(2~{S},3~{S},4~{R},5~{R})-2-hexyl-4,5-bis(oxidanyl)piperidine-3-carboxylic 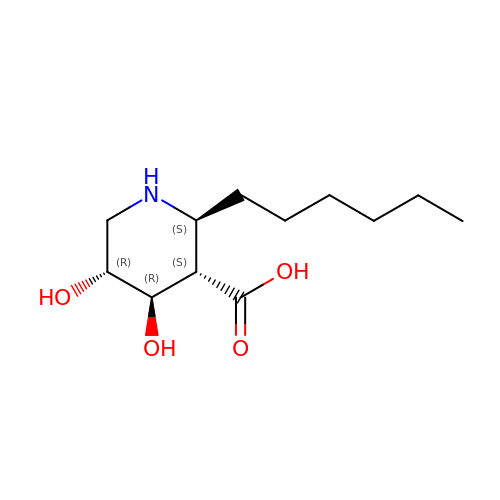acid | C12 H23 N O4 | RRWNAAJMVJWKAM-VLEAKVRGSA-N>[2x]MKVEEILEKALELVIPDEEEVRKGREAEEELRRRLDELGVEYVFVGSYARNTWLKGSLEIDVFLLFPEEFSKEELRERGLEIGKAVLDSYEIRYAEHPYVHGVVKGVEVDVVPCYKLKEPKNIKSAVDRTPFHHKWLEGRIKGKENEVRLLKGFLKANGIYGAEYKVRGFSGYLCELLIVFYGSFLETVKNARRWTRRTVIDVAKGEVRKGEE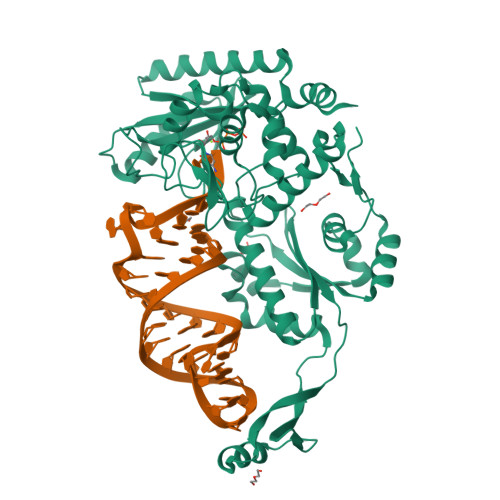FFVVDPVDEKRNVAANLSLDNLARFVHLCREFMEAPSLGFFKPKHPLEIEPERLRKIVEERGTAVFAVKFRKPDIVDDNLYPQLERASRKIFEFLERENFMPLRSAFKASEEFCYLLFECQIKEISRVFRRMGPQFEDERNVKKFLSRNRAFRPFIENGRWWAFEMRKFTTPEEGVRSYASTHWHTLGKNVGESIREYFEIISGEKLFKEPVTAELCEMMGVKDSNSSSVDKLAAALEHHHHHH>GSMATNFDILKRLSNLEKHVFGSKLYD[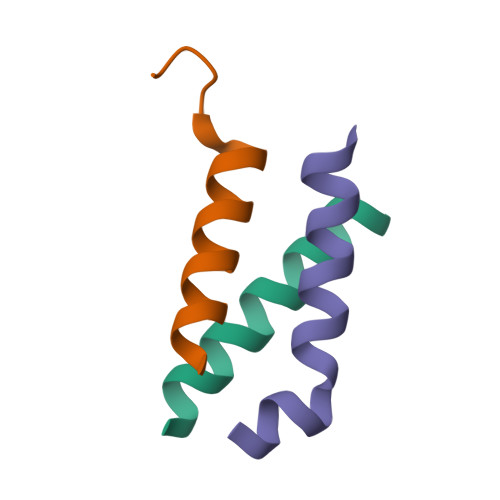9x]>[2x]MGHHHHHHMSPPPAESHIILLI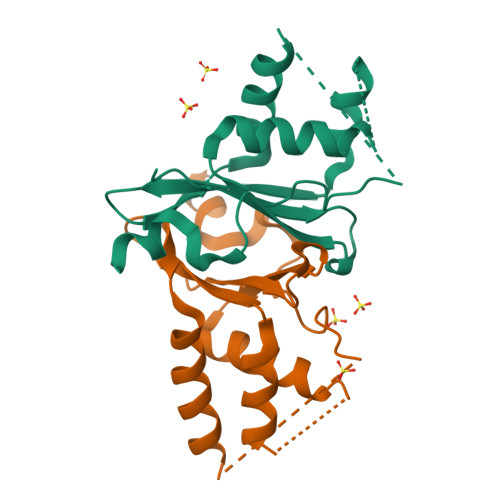QQGSDPKTRIWSDHCSLRSAIEYIVGVYQTNQAVSEKESIDVSRFFNFFDEIYDCVPLVYDRHFRAYIPHEKQWLLHHAQEYLTAARQIPGSSGSSGSSGSSGSSGKYDFSRHCTDYGHSYEWPYFRSLRRES>[4x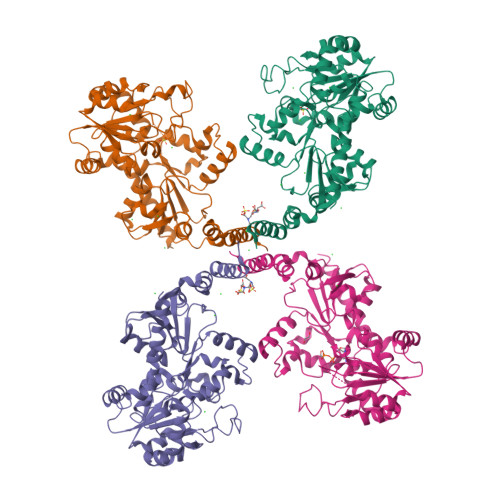]MNKLTIIVTYYNAEEYITGCLESIKQQRTQDFNLIIVNDGSTDQSKKLMDEAIKDYDKNIRFIDLDENSGHAHARNIALEEVETPYFMFLDADDELASYAITFYLEKFNNTDGLIAPIHSFTTQRPQFVDLDRVRVEYFNAKENINSFLRKQSACNIIFRTAIVRAHHIRFNENLNTYVDWSFVLEYMKYVNKFVRIFNFPFYFRGEVYDPFETLTLSEQNFDILFKDYVNSFYDAIKRATNPKVREFIVTKMGNKIANEFEPTRYDINERYQTHKDTLVELSKFLHVHLVKNQKLINKIETILLMNNETDKAFKVNQFRKTLRHVKNIVLRRKNKERSLYDLTDKEDNVKPKTIVFESFGGKNYSDSPKYIYEYMQKYYPNYRYIWSFKNPDKNVVPGSAEKVKRNSAEYYQAYSEASHWVSNARTPLYLNKKENQTYIQTWNGTPLKRLANDMKVVRMPGTTTPKYKRNFNRETSRWDYLISPNRYSTEIFRSAFWMDEERILEIGYPRNDVLVNRANDQEYLDEIRTHLNLPSDKKVIMYAPTWRDDEFVSKGKYLFELKIDLDNLYKELGDDYVILLRMHYLISNALDLSGYENFAIDVSNYNDVSELFLISDCLITDYSSVMFDYGILKRPQFFFAYDIDKYDKGLRGFYMNYMEDLPGPIYTEPYGLAKELKNLDKVQQQYQEKIDAFYDRFCSVDNGKASQYIGDLIHKDIKEQLEHHHHHH>[2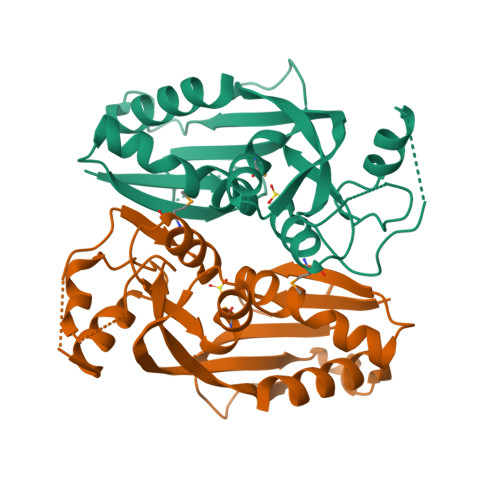x]SNAIQHATASLIQTNTDQELLVVDVTPSFASLWLVPNINDFHQRHPNIRVKILTGDGAVKNIHGESDLHVRCLPLSTHYEYSQLLCEETLLLIGNTNLPKLSDNQAISHYPFIPQTTRPQLWEQFKQENDLECPITYHSVGFEHFYLACEAVRMEKGLALLPDFMAQFSILRGDIQHIGNLKLHSGYGYYVVIPNFRLTSRKVALFHDWLKDKLTHHT N-(4-aminobutyl)acetamide | C6 H14 N2 O 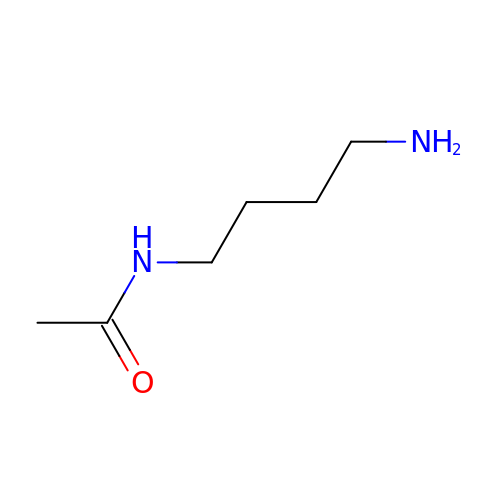| KLZGKIDSEJWEDW-UHFFFAOYSA-N> ADLANGAKVFSGNCAACHMGGGNVV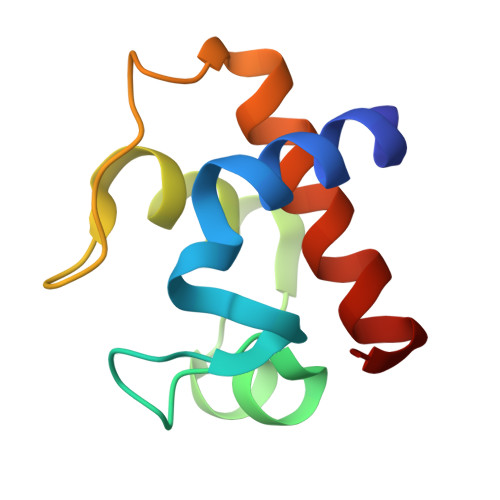MANKTLKKEALEQFGMYSEEAIIYQVQHGKNAMPAFAGRLTDEQIQDVAAYVLDQAAKGWV(3S,4S)-pyrrolidine-3,4-diyl bis(naphthalen-1-ylacetate) | C28 H25 N O4 | 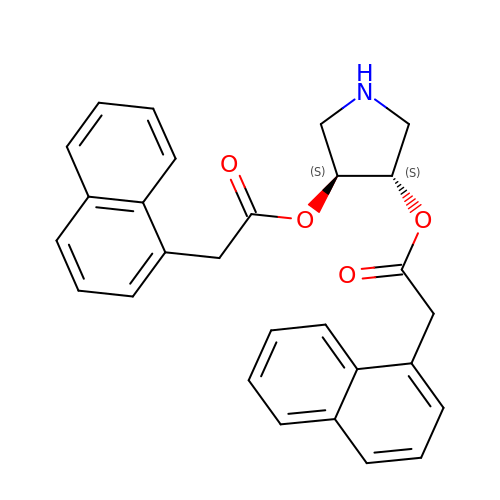ATWKPWWBTFNYMB-UIOOFZCWSA-N>PLGSQFWVTVQRTEAAERCGLHGSYVLRVEAERLTLLTVGAQSQILEPLLSWPYTLLRRYGRDKVMFSFEAGRRCPSGP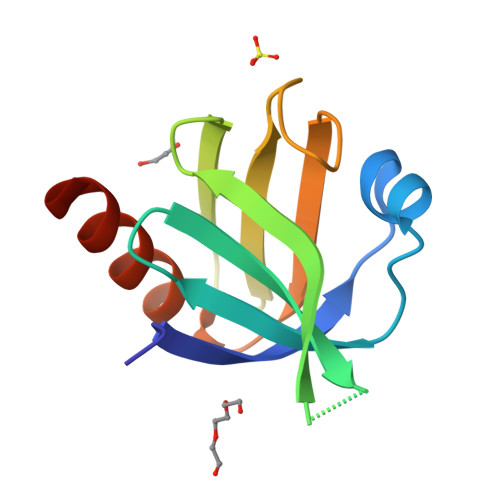GTFTFQTAQGNDIFQAVETAIHRQKAQG[4x]> XVALDXIDISIVLNKIKSQLEESKEWIRR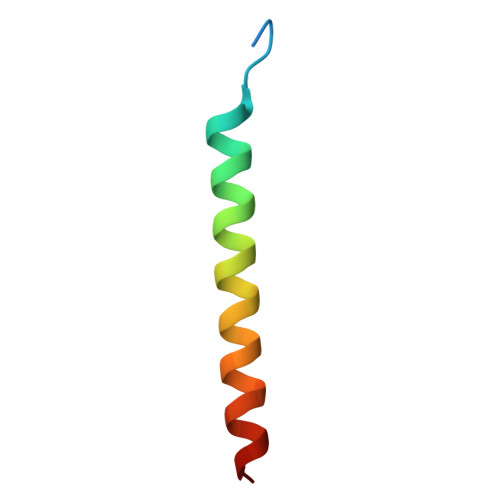SNKILDSIX> GTCTCCAGGCAAC;> 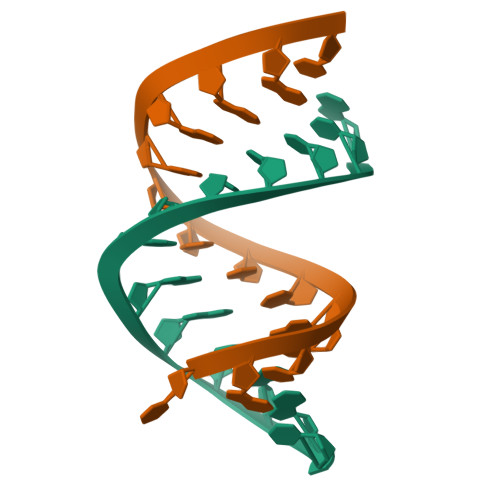UGUUGCCUGGAGAC>[4x]SMGVRKLATIRTAGEITPIAGAEAIECCHVDGWTCVIKKGEFKQGDRGVYFEIDSFIKEDNDRYPMLSKQVIDYEGQRGTRLRTARLRGQLSQGLFLPMDRFPELASNQVGDDVTEILGITKWEPPISTNLSGEILGEFPTFISKTDQERVQNLIPQIEENKGQKFEVTVKLDGSSMTVYRKDDHIGVCGRNWELRETATNAQWHAARRNKMIEGLQFLNRNLALQGAIIGESIQGNLEKLKGQDF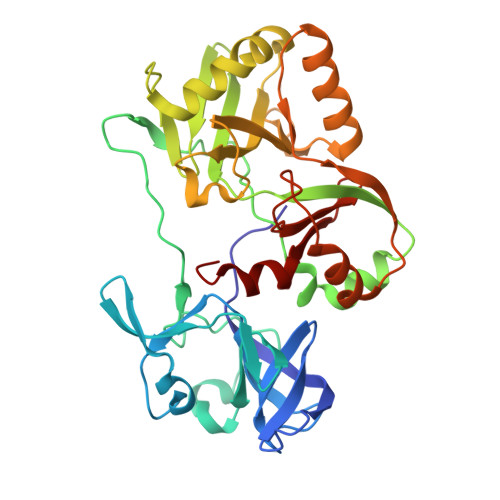YLFDIYDIDKAQYLTPIERQSLVKQLNDNGFTVKHVPILDDLELNHTAEQILAMADGPSLNKNVKREGLVFKRLDGKFSFKAISNAYLEKHKDR>MNNRNHDVLSRMISEKAALHGLLNCLIKEFAIPEGYLRYEWPDEMKGIPPGAYFDGADWKGIPMMIGLPDQLQLFVMVDRRDTFGSQHYLSDVYLRQAQGDWQCPDFEPLVARLLAACEHIAGRKNPELYEQILQSQRLVSAIVSHNGRQRADAPLQHYLQSEQGLWFGHPSHPAPKARLWPAHLGQEQWAPEFQARAALHQFEVPVDGLHIGANGLTPQQVLDGFADQQPASPGHAIICMHPVQAQLFMQDARVQQLLRDNVIRDLGQSGRVASPTASIRTWFIDDHDYFIKGSLNVRITNCVRKNAWYELESTVLIDRLFRQLLDQHADTLGGLVAAAEPGVVSWSPAAAGELDSHWFREQTGGILRENFCRRTGAERSIMAGTLFARGVDLQPMIQTFLRTHYGEALDDNALLYWFDDYQTRLLRPVLSLFFNHGVVMEPHLQNSVLVHQQGRPQQVLLRDFEGVKLTDDLGIRYIDDDIHPRVRQSLLYSREQGWNRIMYC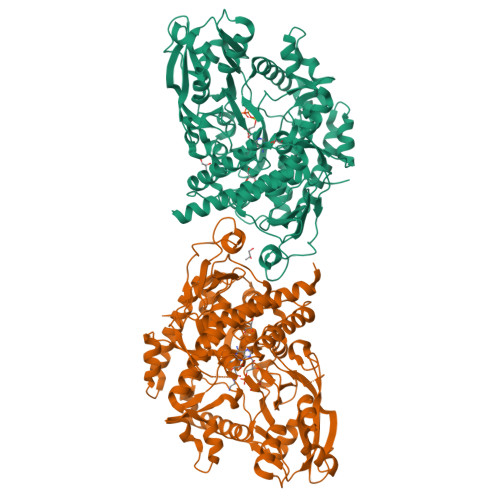LFINHLSETILALSQGRPQLAPLMWRRVQQQLRAIQGELKQPSPELDALIAGHPVACKTNLKVRLAAEADRQASYVRLPSPWGHAVQHGSEVQHDERRHGDVRHEEARHGEVQHG[2x]> MAGASVKVAVRVRPFNSREMSRDSKCIIQMSGSTTTIVNPKQPKETPKSFSFDYSYWSHTSPEDINYASQKQVYRDIGEEMLQHAFEGYNVCIFAYGQTGAGKSYTMMGKQEKDQQGIIPQLCEDLFSRINDTTNDNMSYSVEVSYMEIYCERVRDLLNPKNKGNLRVREHPLLGPYVEDLSKLAVTSYNDIQDLMDSGNKPRTVAATNMNETSSRSHAVFNIIFTQKRHDAETNITTKKVSKISLVDLAGSERADS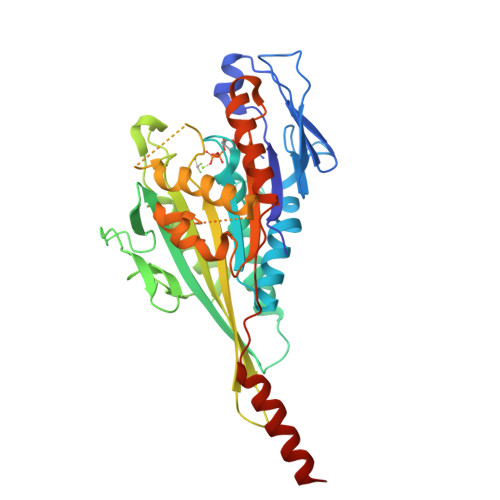TGAKGTRLKEGANINKSLTTLGKVISALAEMDSGPNKNKKKKKTDFIPYRDSVLTWLLRENLGGNSRTAMVAALSPADINYDETLSTLRYADRAKQIRCNAIINEDPNNKLIRELKDEVTRLRDLHHHHHHH> MYQLLSPRTARHARLFRLANNLASSPSGTAGVPKTDGERLLWVNSHVKRNKDIEMSIEEESLRERQLPLKLGENAFTSSAQATHGSLFHFREYPMYPGEYVPAGHNTLSSLRHELRLELTAQSLKEAWMRISGGIYFQSADDYYASVDGLDAEQLGEVLAALFPYLSTYEAQALVQCTLDSISKPMNTASRQLSRTITAEAVGLDNAPGHYTNFLDWMGRLTETRGFKTEHALFQFSRRKFNRDDVRVMFENYKLM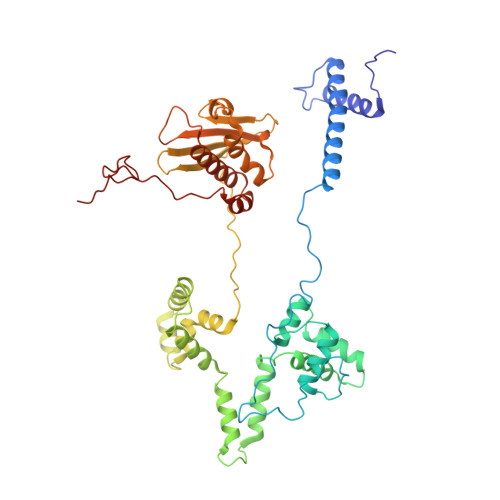SRATLIADSADSYSHFYTVLKDFARKVAGEDSRHQIGVRIDEPEVDAETGIAVGRGCADGEKYQFTALLRENRDHNGAITIMGKPMALVLDNKAWLMEMLLMPFDEANLDYRDFDVHIVLEGHAMPSIANEIAAFALRMSIANALVKLLPLTRIPLKKSGLLSVDRRRERGQFPGYLDGKKVKRKFAKR4-oxopentyl trihydrogen diphosphate | C5 H12 O8 P2 | 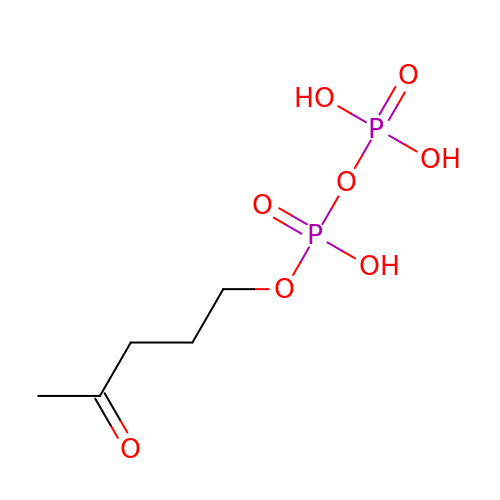KREMOGYKSOVBKI-UHFFFAOYSA-N> AKLGSVYTEGGFVEGVNKKLSLFGDSVDIFKGIPFAAAPKALEKPERHPGWQGTLKAKSFKKRCLQATLTQDSTYGNEDCLYLNIWVPQGRKEVSHDLPVMIWIYGGAFLMGASQGANFLSNYLYDGEEIATRGNVIVVTFNYRVGPLGFLSTGDSNLPGNYGLWDQHMAIAWVKRNIEAFGGDPDQITLFGESAGGASVSLQTLSPYNKGLIKRAISQSGVGLCPWAIQQDPLFWAKRIAEKVGCPVDDTSKMAGCLKITDPRALTLAYKLPLGSTEYPKLHYLSFVPVIDGDFIPDDPVNLYANAADVDYIAGTNDMDGHLFVGMDVPAINSNKQDVTEEDFYKLVSGLTVTKGLRGAQATYEVYTEPWAQDSSQETRKKTMVDLETDILFLIPTKIAVAQHKSHAKSANTYTYLFSQPSRMPIYPKWMGADHADDLQYVFGKPFATPLGYRAQDRTVSKAMIAYWTNFARTGDPNTGHSTVPA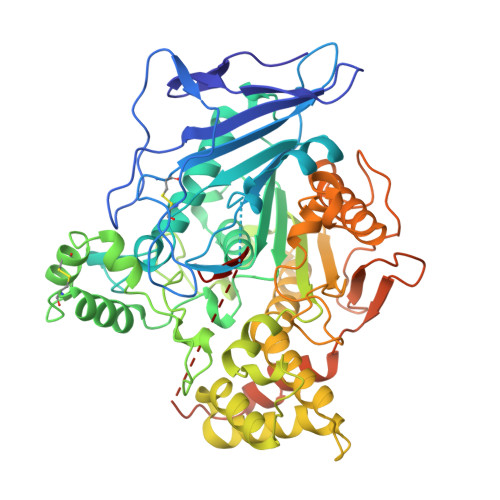NWDPYTLEDDNYLEINKQMDSNSMKLHLRTNYLQFWTQTYQALPTVTSAGASLLPPEDNSQASPVPPADNSGAPTEPSAGDSEVAQMPVVIGF bis(pyrzol-1-yl)acetate scorpionate | C8 H8 N4 O2 | 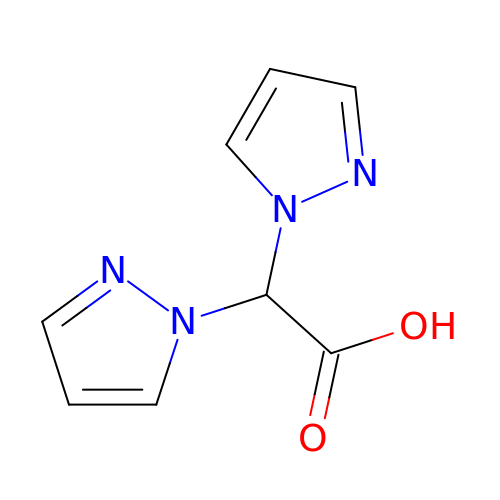NJDSSVBTTVUKHM-UHFFFAOYSA-N> MTAILLACLF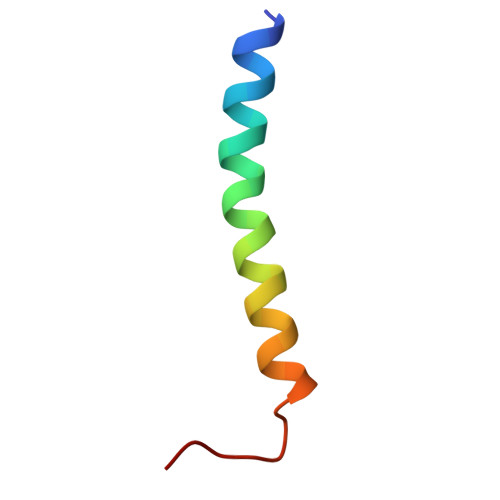VLGGYAALWGIIKFVVANTKDIAAN> MTVPSIVLNDGNSIPQLGYGVFKVPPADTQRAVEEALEVGYRHIDTAAIYGNEEGVGAAIAASGIARDDLFITTKLWNDRHDGDEPAAAIAESLAKLALDQVDLYLVHWPTPAADNYVHAWEKMIELRAAGLTRSIGVSNHLVPHLERIVAATGVVPAVNQIELHPAYQQREITDWAAAHDVKIESWGPLGQGKYDLFGAEPVTAAAAAHGKTPAQAVLRWHLQKGFVVFPKS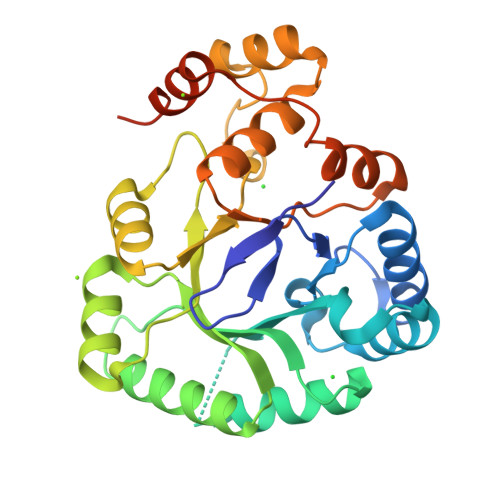VRRERLEENLDVFDFDLTDTEIAAIDAMDPGDGSGRVSAHPDEVD>MLFQQSTRLAQVNCPLGPDVLLLKSLGGGEELGRLFDYQLQLASSDANIDLNQLLGKPMGLSVQLDGGGQRYFHGIVARCSQNIDTGQFASYEVTLRP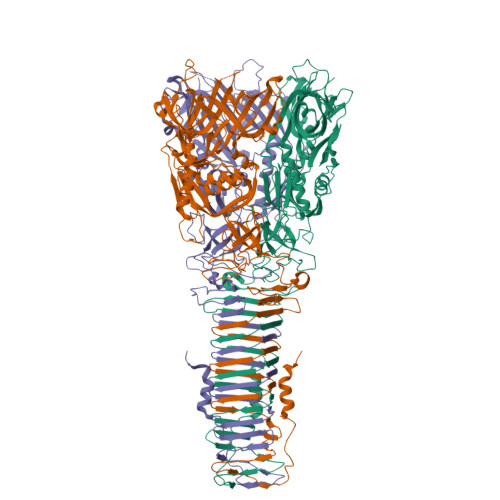WLWLLSRTSDCRIFQNLSIPQIIKQVFRDLGFSDFEDALSRPYREWEYCVQYRETSFDFVSRLMEQEGIYYFFRHEKDRHVVVLADAYGAHSSVPGYASVPYYPRDEQQRERDHMFDWHLAQEVQPGSLELNDYDFQRPSARIDVRSAMPRPHSAGDYPLYDYPGTYVQSSDGEHYAQTRIEALQSLHERIELSGNARGLGVGNLFSLTGFSRQDQNREYLIVSIRYYLVQESLESGAGGGSAQFESHLTCIDAQQSFRPLATTHKPMVQGPQTARVVGPAGEEIWTDQYGRVKVHFHWDRHDQSNENSSCWIRVSQAWAGKNWGSMQIPRIGQEVIVSFLEGDPDRPIITGRVYNAEQTVPYDLPANATQSGMKSRSSKGGSPANFNEIRMEDKKGAEQLYIHAERNQDIVVEVNESHSVGNNRNKSIGHDEYVTIGNKRTRIVQHVDELRVGEKKLDSVGQSYVIEVGERLRLVCGASILELNASGQINLCGVNISVHASADAQINTGGVLHLNNGGGPGTTTEGQGVQGAISAKAKAPFSAPKG[3x]> MRFRDRRHAGALLAEALAPLGLEAPVVLGLPRGGVVVADEVARRLGGELDVVLVRKVGAPGNPEFALGAVGEGGELVLMPYALRYADQSYLE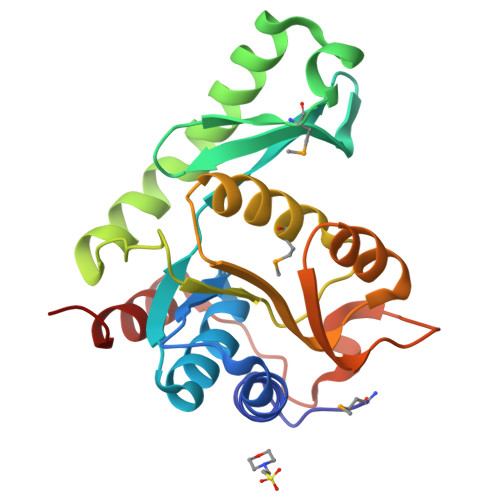REAARQRDVLRKRAERYRRVRPKAARKGRDVVLVDDGVATGASMEAALSVVFQEGPRRVVVAVPVASPEAVERLKARAEVVALSVPQDFAAVGAYYLDFGEVTDEDVEAILLEWAG> EFGHRTLASTPALWASIPCPRSELRLDLVLPSGQSFRWREQSPAHWSGVLADQVWTLTQTEEQLHCTVYRGDLSQASRPTPDELEAVRKYFQLDVTLAQLYHHWGSVDSHFQEVAQKFQGVRLLRQDPIECLFSFICSSNNNIARITGMVERLCQAFGPRLIQLDDVTYHGFPSLQALAGPEVEAHLRKLGLGYRARYVSASARAILEEQGGLAWLQQLRESSYEEAHKALCILPGVGTKVADCICLMALDKPQAVPVDV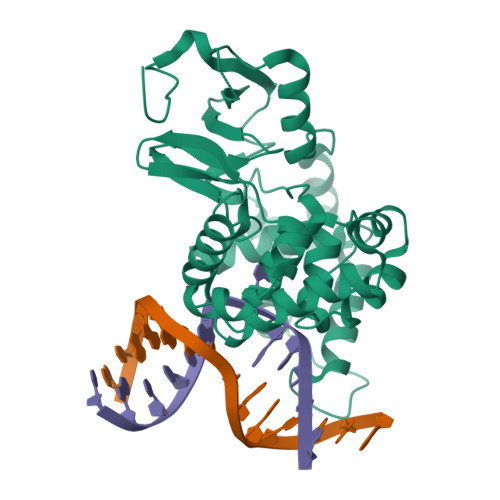HMWHIAQRDYSWHPTTSQAKGPCPQTNKELGNFFRSLWGPYAGWAQAVLFSADLRQ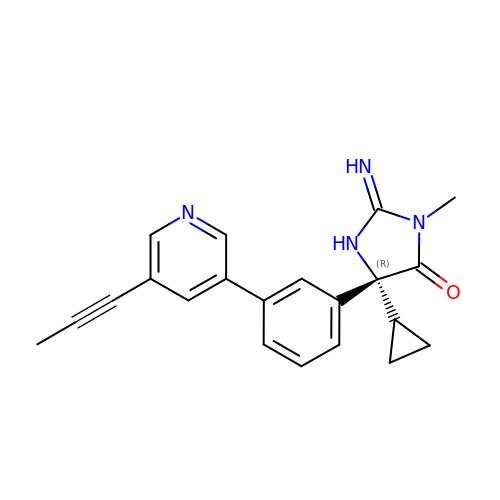(2E,5R)-5-cyclopropyl-2-imino-3-methyl-5-{3-[5-(prop-1-yn-1-yl)pyridin-3-yl]phenyl}imidazolidin-4-one | C21 H20 N4 O | HORHMTMHXZJNQJ-OAQYLSRUSA-N>MTNVFESSPLFLRILLAVLIILLFFYFIFLNYREYKNNNQVKQLNAKVRSLITGHYTDKLKVEDNSDLSELVNNVNDLSEVFRLTHENLAQEKNRLTSILSYMTDGVLATDRSGKITVINDMAQKQLNVTREQALECNILDILDDDSYTYNDLITKTPEIVLTRRDEYDEFITLRIRFALNRRESGFISGLIAVLHDATEQEKEERERRLFVSNVSHELRTPLTSVKSYLEALDDGALTESVAPSFIKVSLDETNRMMRMITDLLSLSRIDNQTSHLDVELTNFTAFMNYILDRFDQIQSQQSTNKVYEIIRDY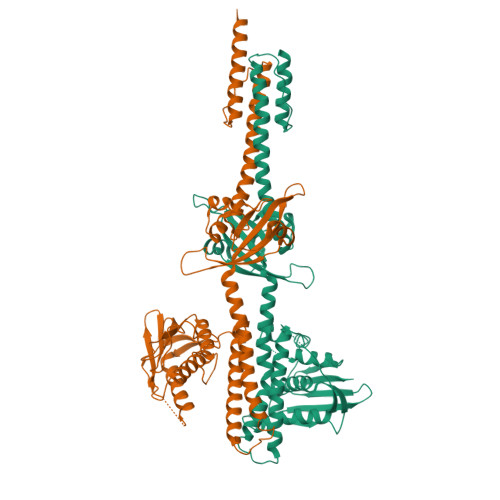PDKSVWIEIDTDKMTQVIDNILNNAIKYSPDGGKVTITMQTTDTQLILSISDQGLGIPKKDLPLIFDRFYRVDKARSRAQGGTGLGLAIAKEIVKQHKGFIWANSEEGEGSTFTIVLPYENDNDAIDEWEEDEDES[2x]>[4x]MAHHHHHHSAARLMAHSIEELAITTIRTLSIDAIEKAKSGHPGMPMGAAPMAYTLWTKFMNHNPANPNWFNRDRFVLSAGHGSMLLYSLLHLSGYDVSMDDLKQFRQWGSKTPGHPEYG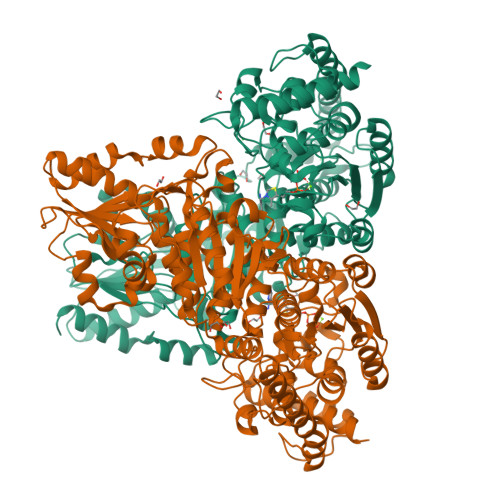HTPGVEATTGPLGQGIAMAVGMAMAERHLAATYNRDGFEIINHYTYAICGDGDLMEGVASEAASLAGHLKLGRLIVLYDSNDISLDGELNLSFSENVAQRFQAYGWQYLRVEDGNNIEEIAKALEEARADLSRPTLIEVKTTIGYGAPNKAGTSGVHGAPLGAQEAKLTKEAYRWTFAEDFYVPEEVYAHFRATVQEPGAKKEAKWNEQLAAYEQAHPELAAQLKRAIEGKLPDGWEASLPVYEAGKSLATRSSSGEVINAIAKAVPQLFGGSADLASSNKTLIKGGGNFFPGSYEGRNVWFGVREFAMGAALNGMALHGGLKVFGGTFFVFSDYLRPAIRLAALMGLPVIYVLTHDSIAVGEDGPTHEPIEQLASLRAMPNLSVIRPADANETAAAWRLALESTDKPTALVLTRQDVPTLAATAELAYEGVKKGAYVVSPAKNGAPEALLLATGSEVGLAVKAQEALAAEGIHVSVISMPSWDRFEAQPKSYRDEVLPPAVTKRLAIEMGASLGWERYVGAEGDILAIDRFGASAPGEKIMAEYGFTVDNVVRRTKALLGK In this study, we solved the structure of SDN1, an exonuclease that initiates miRNA degradation by trimming their 3′ ends to generate unmethylated miRNAs that can be further turned over. Arabidopsis SDN1 and SDN2 belong to the DEDD 3′→5′ exonuclease superfamily, characterized by an active core consisting of three separate sequence motifs with four invariant acidic amino acids (DEDD). The Arabidopsis SDN family belongs to the DEDDh subfamily. Our structural and biochemical studies revealed the structural features of SDN1 in substrate recognition and provided insights on how SDN1 uses its DEDDh catalytic domain and the RRM domain cooperatively to degrade free small RNAs and trim miRNAs in miRNA/target RNA duplexes or miRNAs bound by AGO1.

Full-length, recombinant Arabidopsis SDN1 (residues 2–409) and a 10 nt ssRNA (5′-AGCCCAUUAG-3′) were used in crystallization. However, only the N-terminal domain (NTD; residues 2–137) and the DEDDh catalytic domain (residues 138–300) of SDN1, plus nine nucleotides from the 3′ end of the RNA was clearly observed in the structure. The C-terminal region of SDN1 (residues 301–409) lacked observable density, but was not cleaved during crystallization. In the structure, SDN1 NTD is closely attached to the DEDDh domain through a large interface (1379.2 Å2), and the DEDDh domain interacts with the RNA substrate (530.0 Å2). SDN1 NTD is composed of seven α helices and could not be attributed to any characterized protein family by amino acid sequence or domain architecture. Various hydrophobic interactions and hydrogen bonds (H-bonds) were observed between the NTD and the DEDDh domains, enabling these two domains to form a rather rigid structure. The catalytic pocket of the SDN1 DEDDh domain bound four nucleotides from the 3′ end of the ssRNA substrate. The backbone carboxyl group of M147 and the side chain of Arg185 formed H-bonds with the 2′ and 3′ hydroxyl groups of the 3′ terminal nucleotide G10. His223 and Ser224 on loop 1 (residues 223–225), which connects β4 and α3, formed H-bonds with the phosphate group of A9 and the 2′-OH group on the ribose of U8. In the active center, SDN1 adopted a partially active form, in which two magnesium (Mg) ions were observed at occupancies of 0.57 for MgA and 0.97 for MgB.

> MELKLATAEKQVLDELVKLLQSRDLRGENGNWKEFLHVYDKNADSPSDPSRRSHEDLVQFLTTFKKKEDLQLLKCHANHLLIENLKQESQDEDTPEQMLVRLTVEHPSYSLDYSFKPYSEDWFVSDVGMKMKKVMESTNMVAVDCEMVLCEDGTEGLVRVGVVDRDLKVILDEFVKPNKPVVDYRTDITGITAEDIENASLSVVDIQETLQPFLSTGTILVGHSLNRDLEVLKIDHPKVIDTALVFKYPNTRKLRRPSLNNLCKSILGYEVRKTGVPHDCVHDASAAMKLALAVVEKRVDTTIKPSKEMLEVEKAKLFLHKIPNNVPSEELEQVLSGKFTLDVKQAKTQGRYYCAFALFHSSEDADQAFEHIDGIEMTDSLGLPQKVVIIKLSSGSRASIYVRKMVQDE> MHTLRLFTVLSLLLTSAFTLF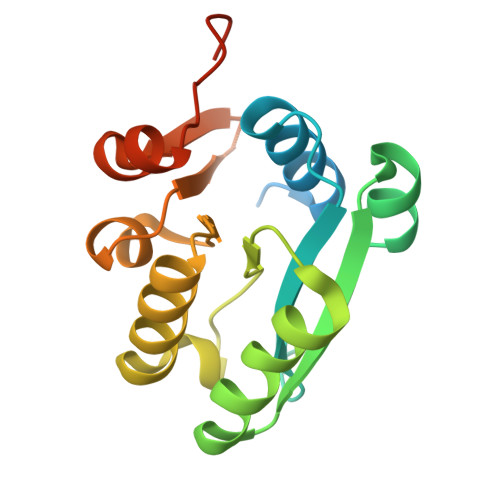PETETEVTPIQQLFLIKELKPGIARIGVIWDKNAANRDEVLPQLQRASAATGIKVVVAEVASLQEVAPQFRTLLRDHQVEALWVLEESGLLGQAAARSFLIKNATQAGMPVFAPSETWLKEGACVTWRKDAEGIRLVVNKAVAEAMGITIPAKYQDRTAFLAMN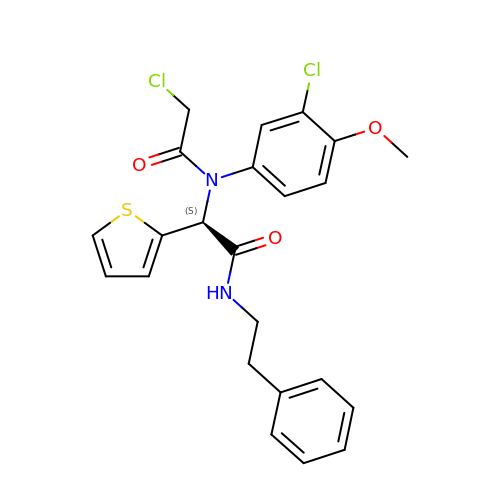(2~{S})-2-[2-chloranylethanoyl-(3-chloranyl-4-methoxy-phenyl)amino]-~{N}-(2-phenylethyl)-2-thiophen-2-yl-ethanamide | C23 H22 Cl2 N2 O3 S | UNVKYJSNMVDZJE-JOCHJYFZSA-N Here we report, in contrast, on a naturally occurring mutation of an otherwise invariant residue in the β-glucosidase BglM-G1 that balances a trade-off between structural stability and enzyme activity. β-glucosidases are enzymes hydrolyzing β-glycosidic bonds in substrates ranging from glycosides, to glucosylated flavonoids, glucosylceramides, and oligosaccharides, releasing nonreducing terminal glucosyl residues (see Ketudat et al. for a comprehensive review). They are also one of the key enzymes in the bioconversion of cellulosic material. The otherwise invariant arginine at position 75 changed to a histidine in this protein, while the other 36 amino acids deemed necessary for the function and structural integrity of members of this protein family remained unchanged. Our data indicate that the natural mutation to histidine at position 75 leads to the loss of an extensive electrostatic network, including a salt bridge in the active site region and implies that evolution of BglM-G1 traded a decrease in thermal stability for improved catalytic efficiency.

We, therefore, re-introduced arginine, replacing the histidine 75 in this enzyme, creating the BglM-G1 variant H75R. This variant showed enzymatic activity and characteristics highly similar to the wild type enzyme with the same pH optimum and buffer preferences, optimal temperature, and comparable substrate specificities. Overall, the side chain and backbone topologies of the amino acid residues in BglM-G1 and its H75R variant were highly similar with an RMSD value of 0.069 Å over 1217 Cα atoms, confirming that the mutation in the active site did not lead to a substantial change in the overall fold. There was, however, a major difference in electrostatic interactions between the mutation site and the active site nucleophile. The naturally occurring histidine at position 75 in BglM-G1 formed only a single hydrogen bond with the backbone oxygen of threonine 116, while arginine at position 75 formed, in addition to hydrogen bond interactions with residues Gln163 and Thr116, a salt bridge with the catalytic nucleophile glutamate at position 349 Fig. 2 CD spectroscopic analysis and X-ray crystal structure of BglM-G1 and its H75R variant. We then determined the melting temperature of both proteins by monitoring changes in ellipticity at 222 nm, while continuously increasing the temperature from 10 to 80 °C. For BglM-G1 the mid-point of transition was at 51.4 °C (324.6 K with a 95% confidence interval between 324.4 and 324.8 K), while the melting temperature of H75R was at 54.9 °C (328.1 K with a 95% confidence interval between 328.9 and 329.2 K). The variant H75R retained its activity at 45 °C over 40 min, while wild type already lost significant activity (p value = 3 × 10−5).

>[3x]MHHHHHHENLYFQGHMKKWGDMFTWGVSTSSYQIEGAANQGGRGPSIWDTFSKIPGAVANGDNGDVACDHYHRYNEDLDLMKWLGVGAYRFSIAWPRVIPSGYGALNKEGMDFYDRLIDGALERGITPWPTLYHWDLPQSLQDKGGWNNRDCAYWFAEYSQKMAEAFSDRLKNWITINEPFCSAWLGHLYGVMAPGIKDLKTGINASHHLLLGHGLATKAIREVSSELKVGITLNFTPAITLGESSEDKLAVELADGFDNRWFGDPVFKAKYPEDIVKAFGKEVPIHPGDMEIISTPLDYLGLNYYFRQTVEYDATAKPLPYKQVTAPNVERTGMGWEVHAQSFTELLERVSKEYKPKEIFITENGSAWDDEVVDGKVDDPNRVSYLERHLDAMFAAKNKGVPISGYFAWSLIDNFEWAYGYAKRFGIIYVDYQTQKRIPKSSAYYYQKRIKES>SIIIPGPNIVPGVNVNRKSKLGRSPAFGAFPVKKQPAVLTQKDDRLEDGIRLDDQLFLKHNKGDMDESWPGLEAAADLYFSKFPTMIHTLTMAAAINGTPNLEGIDMNQAAGYPWNTMGRSRRSLFVQQNGIWLPLPELEAEINKTLEDPYYFYSTFLKDELRPTSKVTLGLTRVVEAAPIHAIIAGRMLLGGLIEYMQANPGKHGSAVGCNPDLHWTKFFFKFCHYPQVFDLDYKCFDATLPSCAFRIVEKHLERLIGDERVTRYIETIRHSRHVFGNETYEMIGGNPSG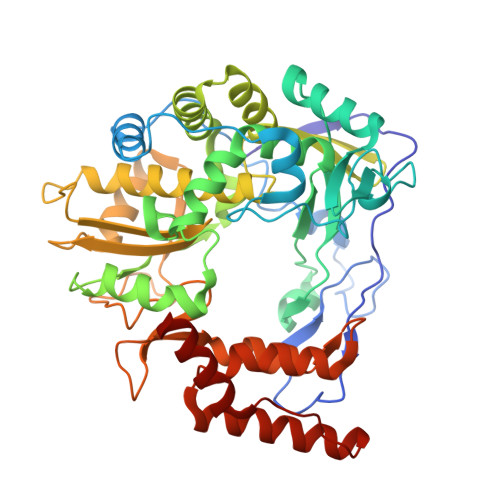CVGTSIINTIINNICVLSALIQHPDFSPESFRILAYGDDVIYGCDPPIHPSFIKEFYDRYTPLVVTPANKTDTFPENSTIYDVTFLKRWFVPDDIRPFYIHPVMDPDTYEQSVMWLRDGDFQDLVTSLCYLAFHSGPKTYDRWCTRVRDQVMKTTGFPPTFLPYSYLQTRWLNLLAA[2x]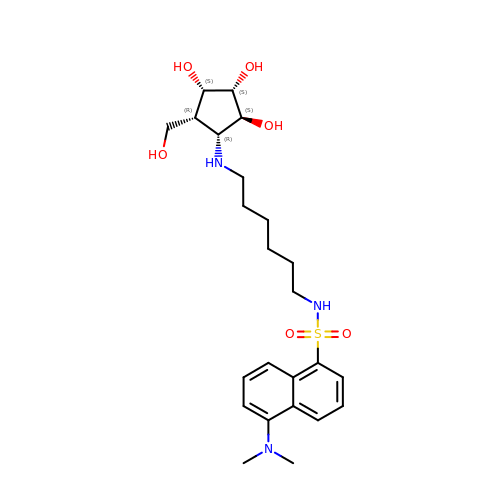5-(dimethylamino)-~{N}-[6-[[(1~{R},2~{R},3~{S},4~{S},5~{S})-2-(hydroxymethyl)-3,4,5-tris(oxidanyl)cyclopentyl]amino]hexyl]naphthalene-1-sulfonamide | C24 H37 N3 O6 S | UQDXIILZCYJPNV-GXWFBMCDSA-N>QVTTEAPAKVVKHSKKQDENIVVNKFKPKEPYVGRCLLNTKITGDDAPGETWHMVFSTEGEVPYREGQSIGIVPDGIDKNGKPHKLRLYSIASSAIGDFGDSKTVSLCVKRLVYTNDAGEVVKGVCSNFLCDLKPGSEVKITGPVGKEMLMPKDPNATVIMLGTGTGIAPFRSFLWKMFFEKHEDYQFNGLAWLFLGVPTSSSLLYKEEFEKMKEKAPENFRLDFAVSREQVNDKGEKMYIQTRMAQYAEELWELLKKDNTFVYMCG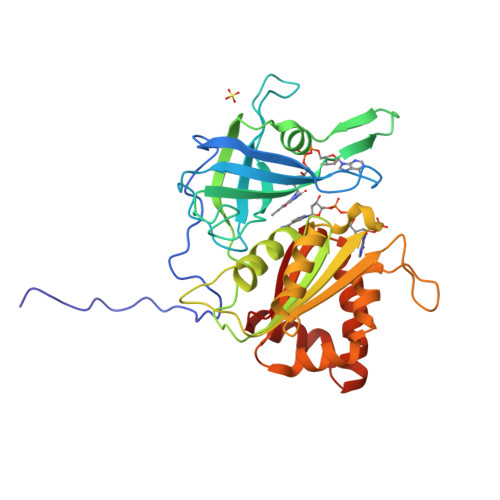LKGMEKGIDDIMVSLAAKDGIDWIEYKRTLKKAEQWNVEVS[2x]P-type ATPases are transmembrane proteins that play a key role in the uphill transport of a wide range of cations across membranes using the energy provided by the hydrolysis of ATP, being crucial for the ion homeostasis in nearly all organisms and for heavy metal detoxification. HMA1 and HMA6 are found in the inner membrane of the chloroplast envelope and HMA8 in the thylakoid membrane. Here, we present two structures of the nucleotide binding domain of HMA6 and HMA8, the former at the highest resolution, obtained for any P-type ATPase structure. The overall structure of HMA6N-AA and HMA8N (respectively) exhibits a twisted, antiparallel β-sheet made of six strands being flanked by two pairs of short α-helices, one on the concave (α1 and α2) and one on the convex (α3 and α4) side of the sheet.

HMA6 represents the main route for copper into the chloroplast, also supplying the Cu/Zn superoxide dismutase, while HMA1 represents a second route for copper, crucial under high light. The initial construct (HMA6N) of the HMA6 N-domain was poorly expressed and required the addition of an N-terminal solubility enhancing tag, which lead to a 15-fold increase in expression. Modifications of the construct and the buffer remained unsuccessful and therefore the construct sequence was analysed using the Surface-Entropy-Reduction prediction (SERp) server for patches of surface residues, which, once mutated, could potentially promote local stability, and the three highest scoring mutants were tested for expression and crystallisation. One of them, the double mutant EE709AA, dubbed construct HMA6N-AA, led, together with a change of the buffer, to an initial crystal hit. A reduction of the protein concentration to 4 mg.mL-1 occasionally led to crystals with a different, more wedge like shape and a different space group (P22121), not showing any more the inter-grown clusters seen initially. These crystals diffracted up to 1.5 Å resolution and contained only two molecules in the AU. Glu709A, in the partially disordered helix α4, points to the solvent and the glutamate of the wild type sequence, when modelled in the structure, clashes with the side chain of Leu705 of the symmetry related chain A*. On the other hand, the side chain of Glu710 points towards the centre of the domain and would clash with Val730 of β6. Several crystal contacts are present between the chains in two axis, while these mutations allowed for a crystal contact in the third axis, between α4 and α4'. An interesting observation in the case of HMA6 is the presence of glutamate 672, not commonly found at this position, pointing to the nucleotide binding cavity and guiding the position of the conserved H645.

>[2x]GASHPVVTEVIIPENPRHNLNDTWSEVEVLMLAAAVESNTTHPVGKAIVKAARARNCQTMKAEDGTFTEEPGSGAVAIVNNKRVTVGTLEWVKRHGATGNSLLALAAHEINNQSVVYIGVDNTLAAVIRFE> GMDAALKRSRSEEPAEILPPARDEEEEEEEGMEQGLEEEEEVDPRIQGELEKLNQSTDDINRRETELEDARQKFRS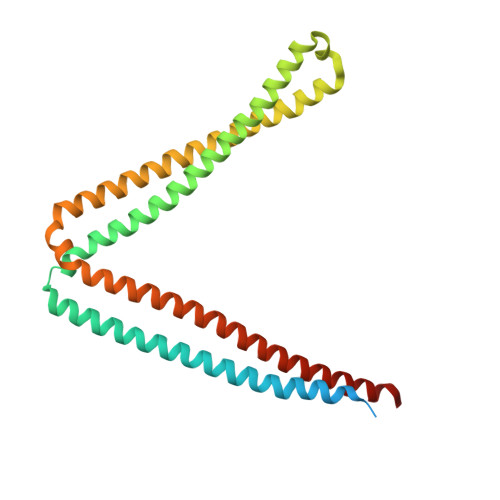VLVEATVKLDELVKKIGKAVEDSKPYWEARRVARQAQLEAQKATQDFQRATEVLRAAKETISLAEQRLLEDDKRQFDSAWQEMLNHATQRVMEAEQTKTRSELVHKETAARYNAAMGRMRQLEKKLKRAINKSKPYFELKAKYYVQLEQLKKTVDDLQAKLTLAKGEYKMALKNLEMISDEIHERRRSSA>[6x]PADAVPAYPFSLPHALDLDPHYAELRRDEPVSRVRLPYGEGTAWLVTRMSDARIVLGDSRFSTAAATDPATPRMFPTPPYPDGVLAQDPPDHTRLRRLVGKAFTARRVEEMRPRVRSLVDSLLDDMVA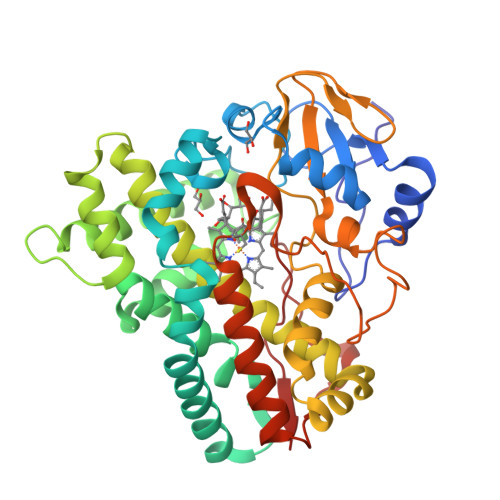HGSPADLVEFLAVPFPVAVICELLGVPLEDRDLFRTFSDAMLSSTRLTAAEIQRVQQDFMVYMDGLVAQRRDAPTEDLLGALALATDNDDHLTKGEIVNMGVSLLIAGHETSVNQITNLVHLLLTERKRYESLVADPALVPAAVEEMLRYTPLVSAGSFVRVATEDVELSTVTVRAGEPCVVHFASANRDEEVFDHADELDFHRERNPHIAFGHGAHHCIGAQLGRLELQEALSALVRRFPTLDLAEPVAGLKWKQGMLIRGLERQIVSW>MAKFPKNFMFGYSWSGFQFEMGLPGSEVESDWWVWVHDKENIASGLVSGDLPENGPAYWHLYKQDHDIAEKLGMDCIRGGIEWARIFPKPTFDVKVDVEKDEEGNIISVDVPESTIKELEKIANMEALEHYRKIYSDWKERGKTFILNLYHWPLPLWIHDPIAVRKLGPDRAPAGWLDEKTVVEFVKFAAFVAYHLDDLVDMWSTMNEPNVVYNQGYINLRSGFPPGYLSFEAAEKAKFNLIQAHIGAYDAIKEYSEK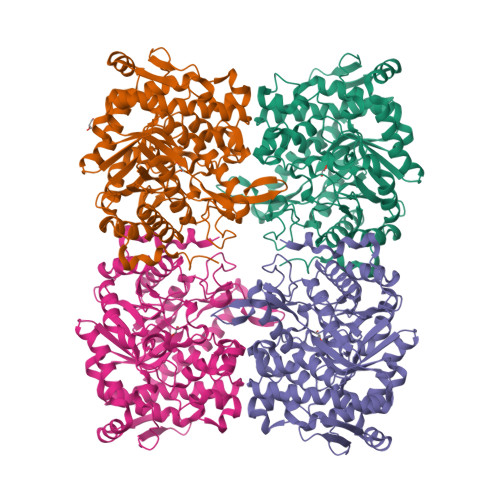SVGVIYAFAWHDPLAEEYKDEVEEIRKKDYEFVTILHSKGKLDWIGVNYYSRLVYGAKDGHLVPLPGYGFMSERGGFAKSGRPASDFGWEMYPEGLENLLKYLNNAYELPMIITENGMADAADRYRPHYLVSHLKAVYNAMKEGADVRGYLHWSLTDNYEWAQGFRMRFGLVYVDFETKKRYLRPSALVFREIATQKEIPEELAHLADLKFVTRK[4x]> GEPLYTEQDLAVNGREGFPNYRIPALTVTPDGDLLASYDGRPTGIDAPGPNSILQRRSTDGGRTWGEQQVVSAGQTTAPIKGFSDPSYLVDRETGTIFNFHVYSQRQGFAGSRPGTDPADPNVLHANVATSTDGGLTWSHRTITADITPDPGWRSRFAASGEGIQLRYGPHAGRLIQQYTIINAAGAFQAVSVYSDDHGRTWRAGEAVGVGMDENKTVELSDGRVLLNSRDSARSGYRKVAVSTDGGHSYGPVTIDRDLPDPTNNASIIRAFPDAPAGSARAKVLLFSNAASQTSRSQGTIRMSCDDGQTWPVSKVFQPGSMSGSTLTALPDGTYGLLYEPGTGIRYANFNLAWLGGICAPFTIPDVALEPGQQVTVPVAVTNQSGIAVPKPSLQLDASPDWQVQGSVEPLMPGRQAKGQVTITVPAGTTPGRYRVGATLRTSAGNASTTFTVTVGLLDQARMS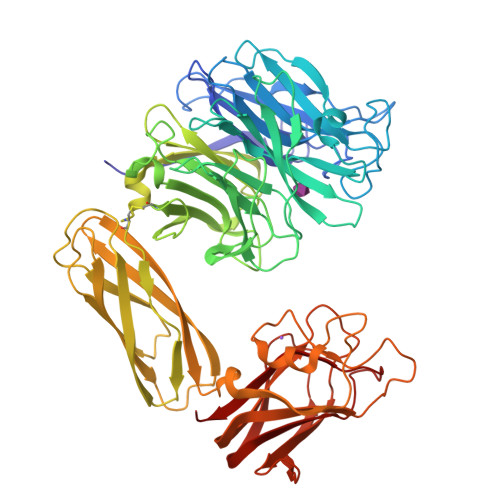IADVDSEETAREDGRASNVIDGNPSTFWHTEWSRADAPGYPHRISLDLGGTHTISGLQYTRRQNSANEQVADYEIYTSLNGTTWDGPVASGRFTTSLAPQRAVFPARDARYIRLVALSEQTGHKYAAVAELEVEGQR>MAENTEPRIGVFVCHCGTNIAGSMSIDDVVNYAKTLPYVAVADQYQYMCSTPGQKKIDDAIKEYNLTGVVVAACSPRLHEPTFRTATKEGGLNPFRFEMANIREQNSWVHMHGMWDEATQKAKDQVRMAVAKAAKLEDLVPKSVPVEKTAMVVGGGVAGMQAALDLASAGIKTYLIERTPTIGGRMSQLDKTFPTLDCSQCILTPKMVDVGRHPNIEMMTYTEVEKVEGYIGNFDVTLRKKARGVLTPTEATAKGIVGGGCNGCGDCSAVCPVIKPNPFEMGMAPRKAIYIYHAQVMPLIYTVDFDSCVKCGLCVEACGDKKAIDLEMQDEFITVKVGTAVLATGYELFPIENKREWGYKQFDNVINALEFERLICASGPTGGHLVRPSDGKTPMKVGFVLCAGSRDNTGIGKPYCSRFCCMYSLKHAHQIMEKIPGAVAYLFYMDIRSFGKMYEEFYYRIQHEGAKFIRGRVANVLEDKETKNLHVFTEDTLLGRPVDVEVDLLVLAAAVQPNEGANELRKKFGVSASQDGWMLEAHPKLNPCGTTTAGVFLAGVCQGPKDIPDTVAQAEGAASAASIPIHMGEVELEPYFAMCIDELCAGCGMCVNLCPYSALSLGEKNGRTVMVVTEAKCKGCGTCGGFCPGGAIKMQHFTTPQIVAQIDAFFAGGEQ[2x];>[2x]MHEYAFFLGCIAPNRYPGCEASAIKTSEKVGIKLLPLKGASCCPAPGAFGSIDLNVWYAMAARNLVLAEEMKKDIALICNGCYKSIWEVNHILKHNDELRDNVNEVLAEIDMQFKGTIDVWHLAELYYDDKVCGVQKIKDSVTTPLSGAKVAAHYGCHLMKPKKERHFGDTENPMWFEELIGALGAEPIQYRNKMQCCGAGGGVRGYDIVHALDITNEKLINIQEAGADAITELCPFCQLQFDRGQIEIKEKFGDVYNIPVLHYNELLGLAQGMSPQDLALDLHAIDCTPFLQKVL;>[2x]MAAKSYNIPELDKKLADRRYHLSDTNPEFTQKILKTSRTIANMCYQCGTCTGSCPSAPRSSYRIRLFMRRCVLGLENEALTDPDLWLCTTCYSCTDRCPRDIAPTDVIMAMRNLAFKRDIVPKNFLQTVQLIYNSGHGVPNNDVNRAARTKLGLPADPPTTHSYPEFVKGIQKIIDHYELKENADRILKGD;> MSENSEIMKYVATTCPYCGVGCTLNLVVSNGKVVGVEPNQRSPINEGKLCPKGVTCWEHIHSPDRLTTPLIKKDGKFIEASWDEALDLVAKNLKVIYDKHGPKGLGFQTSCRTVNEDCYIFQKFARVGFKTNNVDNCARICHGPSVAGLSLSFGSGAATNGFEDALNADLILIWGSNAVEAHPLAGRRIAQAKKKGIQIIAVDPRYTMTARLADTYVRFNPSTHIALANSMMYWIIKEGLEDKKFIQDRVNGFEDLKKTVENYADAEAIHGVPLDVVKDIAFRYAKAKNAVIIYCLGITELTTGTDNVRSMGNLALLTGNVGREGVGVNPLRGQNNVQGACDMGAYPNVYSGYQKCEVAENRAKMEKAWSVTNLPDWYGATLTEQINQCGDEIKGMYILGLNPVVTYPSSNHVKAQLEKLDFLVVQDIFFTETCQYADVILPGACFAEKDGTFTSGERRINRVRKAVNPPGQAKEDIHIISELAAKMGFKGFELPTAKDVWDDMRAVTPSMFGATYEKLERPEGICWPCPTEEHPGTPILHREKFATADGKGNLFGIDYRPPAEVADAEYPFTLMTGRLIFHYHSRTQTDRAADLHREVPESYAQINIEDARRLGIKNNEYIKLKSRRGETTTLARVTDEVAPGVVYMTMHFADGVNNLTNTVLDPMSKMPELKHCAISIEKVGGN;> MAAKGDMLYAWAKDAEIQKKGECGGAVTALLKHALETKMVDAVVAIKKGKDLYDAVPTVITNPEDIIQTAGSLHCGTLLIPKLIKKYLNGAKDMKLAVTCKGCDAMAFYELAKRNQINLDNIIMIGVNCGGSVSPVTARKMISNKFGVDPDTVHKEEIDKGQFIIEYEGGHKGIKIDELEEEGYGRRSNCRRCKMKIPRQADIAAGNWGVIGDKAGKATFLEICSEKGANLVNSAQSKGALEISPADPKGIDIRAKVEKAMFNLGDEWRHRDFEGMGKGKDRLKLMMSESSKCIKCYACVEACPICYCIECSTKKPWYIAPGVLPTSFMFHLIRFA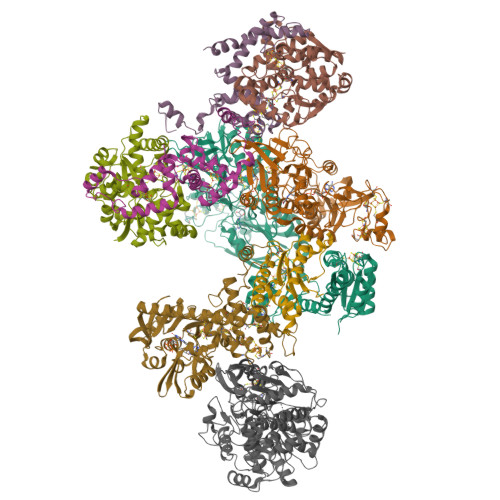HVSDSCINCGQCEELCPMEIPNALFMHSQQVEIEKMFGHIPGQDMTPPIHAFVEEKAERARLDATGTDSIYTNIFTDE;> MADDWKPQILAIICNWCSYAGADLAGGARIQYPPTVRAIRVMCTGRVDMLFILKAFVEGADGVLVSGCHFGDCHYLEGNYKAAKRMFMIKNLLRNIGLDDRRFRMTFVSASEGAKWGMVMEDVTNTIKELGPSPIKEFKK>[2x]MYGKIIFVLLLSEIVSISASSTTGVAMHTSTS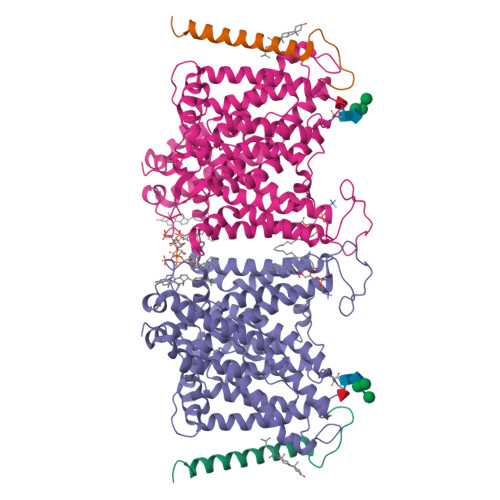SSVTKSYISSQTNDTHKRDTYAATPRAHEVSEISVRTVYPPEEETGERVQLAHHFSEPEITLIIFGVMAGVIGTILLISYGIRRLIKKSPSDVKPLPSPDTDVPLSSVEIENPETSDQ;>[2x]MEELQDDYEDMMEENLEQEEYEDPDIPESQMEEPAAHDTEATATDYHTTSHPGTHKVYVELQELVMDEKNQELRWMEAARWVQLEENLGENGAWGRPHLSHLTFWSLLELRRVFTKGTVLLDLQETSLAGVANQLLDRFIFEDQIRPQDREELLRALLLKHSHAGELEALGGVKPAVLTRSGDPSQPLLPQHSSLETQLFCEQGDGGTEGHSPSGILEKIPPDSEATLVLVGRADFLEQPVLGFVRLQEAAELEAVELPVPIRFLFVLLGPEAPHIDYTQLGRAAATLMSERVFRIDAYMAQSRGELLHSLEGFLDCSLVLPPTDAPSEQALLSLVPVQRELLRRRYQSSPAKPDSSFYKGLDLNGGPDDPLQQTGQLFGGLVRDIRRRYPYYLSDITDAFSPQVLAAVIFIYFAALSPAITFGGLLGEKTRNQMGVSELLISTAVQGILFALLGAQPLLVVGFSGPLLVFEEAFFSFCETNGLEYIVGRVWIGFWLILLVVLVVAFEGSFLVRFISRYTQEIFSFLISLIFIYETFSKLIKIFQDHPLQKTYNYNVLMVPKPQGPLPNTALLSLVLMAGTFFFAMMLRKFKNSSYFPGKLRRVIGDFGVPISILIMVLVDFFIQDTYTQKLSVPDGFKVSNSSARGWVIHPLGLRSEFPIWMMFASALPALLVFILIFLESQITTLIVSKPERKMVKGSGFHLDLLLVVGMGGVAALFGMPWLSATTVRSVTHANALTVMGKASTPGAAAQIQEVKEQRISGLLVAVLVGLSILMEPILSRIPLAVLFGIFLYMGVTSLSGIQLFDRILLLFKPPKYHPDVPYVKRVKTWRMHLFTGIQIICLAVLWVVKSTPASLALPFVLILTVPLRRVLLPLIFRNVELQCLDADDAKATFDEEEGRDEYDEVAMPV>LQELRRELEELSVGSD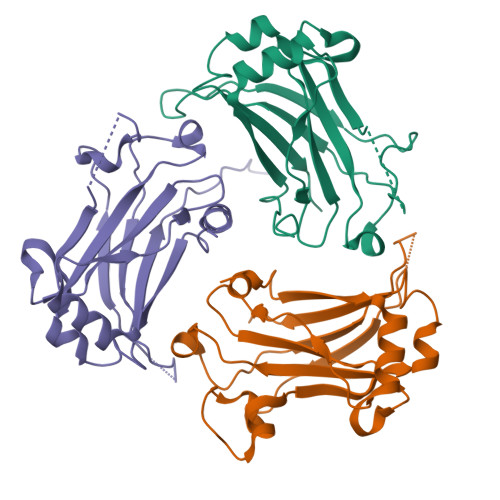GVLIWKIGSYGRRLQEAKAKPNLECFSPAFYTHKYGYKLQVSAFLNGNGSGEGTHLSLYIRVLPGAFDNLLEWPFARRVTFSLLDQSDPGLAKPQHVTETFHPDPNWKNFQKPGTWRGSLDESSLGFGYPKFISHQDIRKRNYVRDDAVFIRAAVELPRLEHHHHHH[3x]Mal, which is also identified as the TIR domain-containing adaptor protein (TIRAP), is essential for the TLR4 and TLR2 signaling pathways. Mal acts as a bridge adaptor to recruit the MyD88 molecule to the activated TLR4 dimer on the plasma membrane. The C-terminus (residues 80–221) of Mal, referred to as Mal-TIR, is the TIR domain and is required for interactions with TLR4, TLR2 and MyD88. The overall structure of Mal-TIR consists of a central five-stranded parallel sheet (βA-βE) surrounded by four helices (αA, αC-αE) on both sides.

The most interesting single nucleotide polymorphism (SNP) is S180L in Mal. Heterozygous carriers of this variant are protected against some infectious diseases, including bacteremia, invasive pneumococcal disease, malaria and atopic dermatitis. The genetic variant Mal S180L has been reported to provide protection against various infectious diseases in different ethnic groups in a number of countries. To further understand the molecular mechanism underlying these associations in the Mal-TIR mutants D96N and S180L, we determined the crystal structures of these mutants. These structures showed that neither mutation interferes with the overall structure of the TIR domain. In our crystal structure of Mal S180L, this mutation changed a negatively charged surface to a positively charged surface and a hydrophilic surface to a hydrophobic surface, thus forming a continuous hydrophobic surface. This hydrophobic patch may play a role in interactions of other binding partners because the S180L mutant is capable of binding normally with MyD88-TIR and TLR4-TIR. The crystals of Valkov et al. were obtained in a solution containing 10–12% PEG 10,000, 5% PEG 3,350, 0.2 M NaCl, 0.1 M Tris-HCl (pH 7.3), and 20 mM DTT and diffracted to 3.0 Å resolution, while the crystals for this study were grown in n-cyclohexyl-2-aminoethanesulfonic acid (CHES) (pH 9.5), 150–300 mM NaCl, 10–20% glycerol and 10 mM DTT and diffracted to 2.4 Å resolution. Both structures of Mal-TIR identified the unusually long AB loop instead of the helix αB and BB loops in other known TIR domains and included two disulfide bonds (residues C89–C134 and C142–C174) and an additional DTT molecule that linked two cysteine residues, Cys91 and Cys157.

> GPGSSRWSKDYDVCVCHSEEDLVAAQDLVSYLEGSTASLRCFLQLRDATPGGAIVSELCQALSSSHCRVLLITPGFLQDPWCKYQMLQALTEAPGAEGCTIPLLLGLSRAAYPPELRFMYYVDGRGPDGGFRQVKEAVMRYLQTLS> KRIVACDDPDFLTSYFAHSRLHHLSAWKANLKDKFLNENIHKYTKITDKDTYIIFHIDFDCFFATVAYLCRSSSFSACDFKRDPIVVCHGTKNSDIASCNYVARSYGIKNGMWVSQAEKMLPNGIKLISLPYTFEQFQLKSEAFYSTLKRLNIFNLILPISIDEAVCVRIIPDNIHNTNTLNARLCEEIRQEIFQGTNGCTVSIGCSDSLVLARLALKMAKPNGYNITFKSNLSEEFWSSFKLDDLPGVGHSTLSRLESTFDSPHSLNDLRKRYTLDALKASVGSKLGMKIHLALQGQDDEESLKILYDPKEVLQRKSLSIDINWGIRFKNITQVDLFIERGCQYLLEKLNEINKTTSQITLKLMRRCKDAPIEPPKYMGMGRCDSFSRSSRLGIPTNEFGIIATEMKSLYRTLGCPPMELRGLALQFNKLVDV

Rev1 is thus unique among TLS polymerases in its protein-template-directed mechanism of DNA synthesis and its specificity in incorporating C opposite template dG. That is, the enzyme embraces the template–primer DNA with its palm (residues 356–365, 438–536), fingers (residues 366–437), and thumb (537–603) domains as well as the PAD (polymerase associated domain; residues 621–738), which is unique to Y-family polymerases. An α-helical substructure at the N terminus, an N-digit (residues 305–355) augments this embrace and makes critical interactions with the incoming dCTP and the templating base. The ability of Rev1 to evict these bulky adducts from the DNA helix and to position Arg324 as the surrogate protein template residue allows for the incorporation of a correct C opposite these stereoisomers, consistent with the previous in vitro studies.

The structure of the 10S (+)-trans-BP-dG-containing ternary complex was obtained by molecular replacement using the 10R (+)-cis-BP complex as a search model and refined to 1.85 Å resolution and Rwork/free 17.0%/20.8%, respectively. The thumb and the PAD are positioned on opposite sides of the DNA duplex and are connected by a long helical linker. The incoming dCTP does not pair with templating 10S (+)-trans-BP-dG; instead, Arg324 (from the N-digit) acts as a “surrogate” residue and makes a set of complementary hydrogen bonds with the cytosine base of the incoming dCTP as observed previously in the unmodified structure. The modified dG is evicted from the DNA helix by Leu325 from the N-digit. Consequently, the BP moiety is located in the major groove of the DNA. The 10S (+)-trans-BP moiety is placed in the solvent-filled space between the PAD and the template–primer DNA helix. The low average B-factors for atoms of the BP and the modified dG moieties (32.6 and 20.8 Å2, respectively) are close in value to the B-factors of the atoms of protein-bound portion of the DNA duplex (24.5 Å2) and indicate the well-ordered alignment of the adduct. Interestingly, the BP pyrenyl ring system points towards the 5′-direction of the modified strand. This is made possible by the modified dG base tilting by ~ 44° in the 3′-direction to create room for the BP moiety to extend in the opposite direction, as shown in Fig. 3a, b. The hydroxyl groups at the C9 (C9-OH) and C8 (C8-OH) of the BP face away from the W–C edge of dG. 2-dG adduct differs in how it is accommodated in the Rev1 active site versus free DNA, the torsion angles α′ and β′ defining the local conformation of the carcinogen-DNA linkage site are similar in both cases and are in the most favorable range for a 10S (+)-trans-BP-dG-modified nucleoside, namely α′ = 180 ± 40°, β′ = -90 ± 40°51.>[2x]GAMGGEEVSEEGFQIPATITERYKVGRTIGDGNFAVVKECVERSTAREYALKIIKKSKCRGKEHMIQNEVSILRRVKHPNIVLLIEEMDVPTELYLVMELVKGGDLFDAITSTNKYTERDASGMLYNLASAIKYLHSLNIVHRDIKPENLLVYEHQDGSKSLKLGDFGLATIVDGPLYTVCGTPTYVAPEIIAETGYGLKVDIWAAGVITYILLCGFPPFRGSGDDQEVLFDQILMGQVDFPSPYWDNVSDSAKELITMMLLVDVDQRFSAVQVLEHPWVND

Doublecortin-like kinase 1 (DCLK) is a microtubule-associated serine/threonine kinase that contains two tandem doublecortin (DCX) domains on its N-terminus. The C-terminal kinase domain shows high resemblance to Ca2+/calmodulin-dependent protein kinase 1 (CaMKI) domain. Between the domains is a flexible PEST linker region rich in proline, glutamate, serine, and threonine and harboring multiple phosphorylation sites. Given the functional attributes of Doublecortin-like kinase 1 (DCLK1) in tumor growth, invasion, metastasis, cell motility, and tumor stemness, it is emerging as a therapeutic target in gastrointestinal cancers.

To provide reliable structural information for rational design of inhibitors and to further explore the mechanism of action of ruxolitinib, the crystal structure of the DCLK1 kinase domain in the complex of ruxolitinib (DCLK1KD·Ruxolitinib) was determined at 2.1 Å resolution by soaking a threefold molar excess of ruxolitinib into the AMPPNP-complexed DCLK1 crystal for substitution. Expectedly, the structure adopts the overall kinase domain architecture, with an N-lobe and a C-lobe, where the inter-lobe cleft represents the ATP binding site, which is occupied by the small molecule inhibitor, ruxolitinib. In accordance with the previously reported DCLK1 kinase domain structures, the DCLK1KD·Ruxolitinib structure displays an active-state conformation with a DFG-in conformation where the side chain of Asp533 is positioned toward the ATP-binding site and the Phe534 residue is in contact with the αC-helix of the N-terminal lobe. In addition, an inward disposition of the αC-helix positions Glu436 on the helix to form a salt bridge with strictly conserved Lys419. However, the DCLK1KD·Ruxolitinib structure shows dimer formation not mediated by any ligand mimicking the phosphorylated form, but still retains active conformation (left). In contrast, the β3-αC loop of the dimer structure of DCLK1KD·Ruxolitinib is flipped over by the large movement of Arg427Nη (18.4 Å), resulting in the concomitant shift of Glu515Oε (4.9 Å). In details, the pyrrolopyrimidine ring of ruxolitinib is sandwiched between Val404 and Ala417 of N-lobe and Leu518 of C-lobe via hydrophobic contacts and is oriented toward the hinge region to form two hydrogen bonds with the main chains of Glu466 and Val468 with the distances of 2.9 Å and 3.2 Å, respectively. The nitrile on the propanenitrile group confers a significant affinity for DCLK1, making an intensive network of interactions with the main chains of Glu515 and Asn516 on the C-lobe, which is in a similar position with the interactions for the ribose sugar of AMPPNP in the DCLK15JZJ·AMPPNP structure and with the side chains of invariant Lys419 and Glu436 on the N-lobe via a water molecule. The cyclopentyl group of ruxolitinib contributes to the tight binding by occupying a hydrophobic groove underneath a conserved glycine-rich loop, or P-loop, which connects the β1 and β2 strands.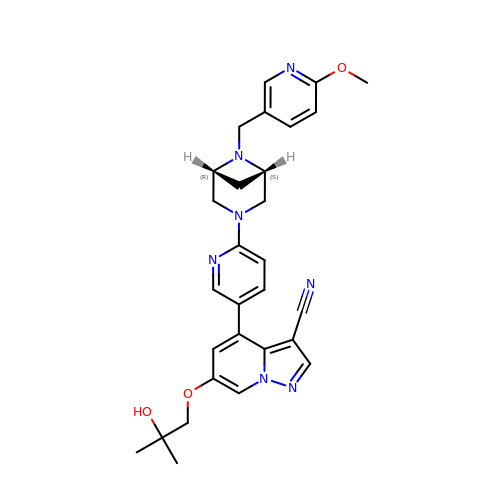Selpercatinib | C29 H31 N7 O3 | XIIOFHFUYBLOLW-ZRZAMGCNSA-N> DAAPGASKLRAVLEKLKLSRDDISTAAGMVKG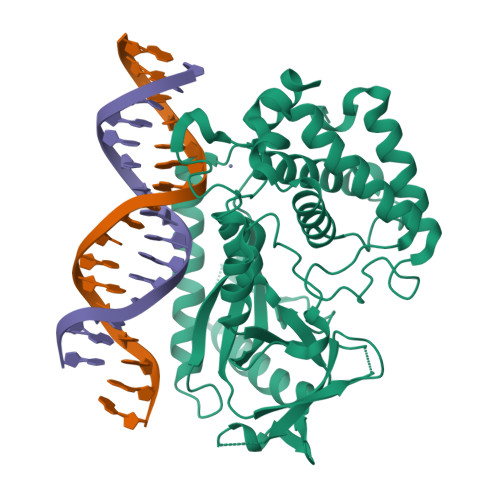VVDHLLLRLKCDSAFRGVGLLNTGSYYEHVKISAPNEFDVMFKLEVPRIQLEEYSNTRAYYFVKFKRNPKENPLSQFLEGEILSASKMLSKFRKIIKEEINDIKDTDVIMEAERGGSPAVTLLISEKISVDITLALESKSSWPASTQEGLRIQNWLSAKVRKQLRLKPFYLVPKHAKEGNGFQEETWRLSFSHIEKEILNNHGKSKTCCENKEEKCCRKDCLKLMKYLLEQLKERFKDKKHLDKFSSYHVKTAFFHVCTQNPQDSQWDRKDLGLCFDNCVTYFLQCLRTEKLENYFIPEFNLFSSNLIDKRSKEFLTKQIEYERNNEFPVFDEF> XQLAL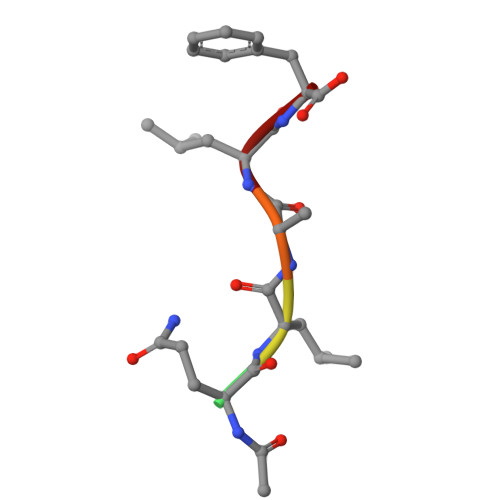F> MVRKMRIAVIDYDKCNPDKCGHFLCERVCPVNRMGGEAIIIDEENYKPIIQEASCTGCGICVHKCPFNAISIVNLPEQLDEDCVHRYGVNAFVLYRLPIVKDGMVVGIVGPNGTGKTTAVKILAGQLIPNLCEDNDSWDNVIRAFRGNELQNYFERLKNGEIRPVVKPQYVDLLPKAVKGKVRELLKKVDEVGKFEEVVKELELENVLDRELHQLSGGELQRVAIAAALLRKAHFYFFDEPSSYLDIRQRLKVARVIRRLANEGKAVLVVEHDLAVLDYLSDVIHVVYGEPGVYGIFSKPKGTRNGINEFLQGYLKDENVRFRPYEIRFTKLSERVDVERETLVEYPRLVKDYGSFKLEVEPGEIRKGEVIGIVGPNGIGKTTFVKMLAGVEEPTEGKVEWDLTVAYKPQYIKAEYEGTVYELLSKIDSSKLNSNFYKTELLKPLGIIDLYDRNVEDLSGGELQRVAIAATLLRDADIYLLDEPSAYLDVEQRLAVSRAIRHLMEKNEKTALVVEHDVLMIDYVSDRLIVFEGEPGRHGRALPPMGMREGMNRFLASVGITFRRDPDSGRPRANKEGSVKDREQKARGEYYYA

In Eukarya and Archaea, the ATP binding cassette (ABC) protein ABCE1 catalyses the essential step of ribosome recycling by splitting the ribosome into its small 40/30S and large 60/50S subunits. ABCE1 is equipped with two nucleotide-binding domains (NBDs) oriented in a head-to-tail fashion and connected via hinge 1 and 2 region. Furthermore, it contains a unique N-terminal FeS cluster domain, aligned by two diamagnetic [4Fe–4S]2+ clusters. Hence, ABCE1 emerges as the missing link between termination and initiation by potentially coordinating the re-initiation via the released 40/30S·ABCE1 complex, named post-recycling complex (PRC), where ABCE1 remains bound after ribosome splitting until ATP hydrolysis has occurred.

Using a homogeneously purified population of the 1-MDa PRC composed of 16S ribosomal RNA (rRNA), 28 ribosomal (r-)proteins and ABCE1 stably arrested by non-hydrolysable AMP-PNP, we mapped the position of ABCE1 within this multisubunit ribonucleoprotein particle by means of XL-MS. To provide a second, independent line of evidence for the position of ABCE1 and the extreme structural reorganization of the FeS cluster domain in the PRC, we analysed the archaeal 30S·ABCE1·AMP-PNP complex by cryo-EM. In spite of the facts that archaeal 30S ribosomal particles were up to now not accessible to cryo-EM analyses and occupancy was low, we resolved the structural architecture of the PRC by a low-resolution cryo-EM reconstruction, in which, indeed, an extra density near rRNA helix 44 (h44) and S12 was observed. While the two NBDs fit into the body part of the ABCE1 density as shown in the pre-splitting state, confirming the cross-links between the HLH region and the ribosomal subunit S24e, there was no visible density for the FeS cluster domain in the pre-splitting position. Notably, with a 160-degree rotation of the FeS cluster domain from the pivot point (proline 76), the extra density near S12 and h44 could be easily positioned in a way that explains the cross-link data described above. The orientation of the FeS cluster domain is based on positioning lysine 60 of ABCE1 and lysine 40 of S12 at a Cα–Cα distance of 17.5 Å, using cross-linker and lever length as restraints. Because of this conformation change, the Cα–Cα distance between these highly conserved lysines in Archaea, yeast and human is reduced from 59.5 Å in the pre-splitting state to 17.5 Å in the post-recycling state. Lysines 133, 136, 141, 153 and 192 of ABCE1, most of them residing in the helix–loop–helix (HLH) region (aa 132-161), form cross-links with lysine 113 or 119 of the ribosomal subunit S24e. In addition, lysine 60 of the FeS cluster domain (ABCE1) cross-links with lysine 40 of the ribosomal protein S12. On NBD closure, the FeS cluster domain, anchored to NBD1 via a two β-strand lever-arm, swings out of the NBD cleft and converges towards the 30S subunit to occupy a cleft between the S12 r-protein and rRNA (h44) of the small ribosomal subunit.> MSQSNRELVVDFLSYKLSQKGYSWSQFSDVEENRTEAPEETEPERETPSAINGNPSWHLADSPAVNGATGHSSSLDAREVIPMAAVKQALREAGDEFELRYRRAFSDLTSQLHITPGTA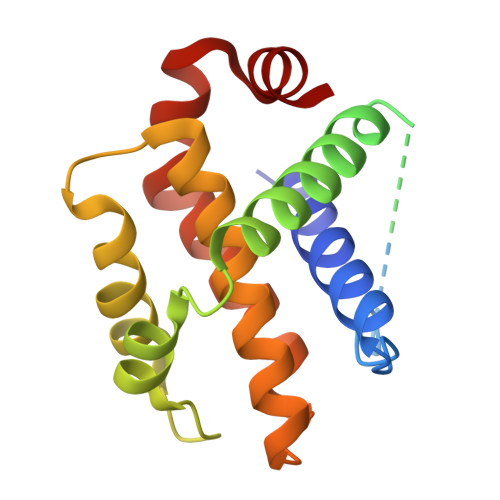YQSFEQVVNELFRDGVNWGRIVAFFSFGGALCVESVDKEMQVLVSRIASWMATYLNDHLEPWIQENGGWDTFVDLYG> ELPNYLVTLPARLNFPSVQKVCLDLSPGYSDVKFTVTLETKDKTQKLLEYSGLKKRHLHCISFLVPPPAGGTEEVATIRVSGVGNNISFEEKKKVLIQRQGNGTFVQTDKPLYTPGQQVYFRIVTMDSNFVPVNDKYSMVELQDPNSNRIAQWLEVVPEQGIVDLSFQLAPEAMLGTYTVAVAEGKTFGTFSVEEYVLPKFKVEVVEPKELSTVQESFLVKICCRYTYGKPMLGAVQVSVCQKANTYWYREVEREQLPDKCRNLSGQTDKTGCFSAPVDMATFDLIGYAYSHQINIVATVVEEGTGVEANATQNIYISPQMGSMTFEDTSNFYHPNFPFSGKIRVRGHDDSFLKNHLVFLVIYGTNGTFNQTLVTDNNGLAPFTLETSGWNGTDVSLEGKFQMEDLVYNPEQVPRYYQNAYLHLRPFYSTTRSFLGIHRLNGPLKCGQPQEVLVDYYIDPADASPDQEISFSYYLIGKGSLVMEGQKHLNSKKKGLKASFSLSLTFTSRLAPDPSLVIYAIFPSGGVVADKIQFSVEMCFDNQVSLGFSPSQQLPGAEVELQLQAAPGSLCALRAVDESVLLLRPDRELSNRSVYGMFPFWYGHYPYQVAEYDQCPVSGPWDFPQPLIDPMPQGHSSQRSIIWRPSFSEGTDLFS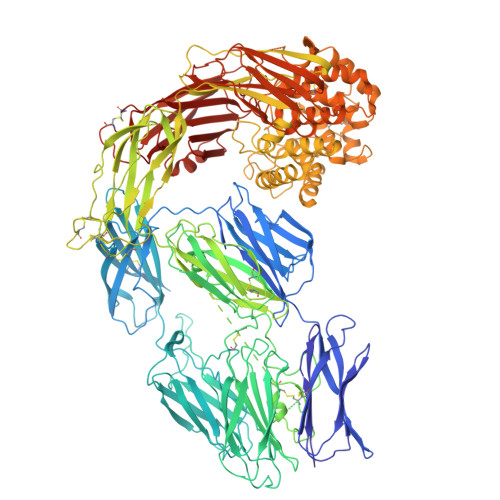FFRDVGLKILSNAKIKKPVDCSHRSPEYSTAMGAGGGHPEAFESSTPLHQAEDSQVRQYFPETWLWDLFPIGNSGKEAVHVTVPDAITEWKAMSFCTSQSRGFGLSPTVGLTAFKPFFVDLTLPYSVVRGESFRLTATIFNYLKDCIRVQTDLAKSHEYQLESWADSQTSSCLCADDAKTHHWNITAVKLGHINFTISTKILDSNEPCGGQKGFVPQKGRSDTLIKPVLVKPEGVLVEKTHSSLLCPKGKVASESVSLELPVDIVPDSTKAYVTVLGDIMGTALQNLDGLVQMPSGCGEQNMVLFAPIIYVLQYLEKAGLLTEEIRSRAVGFLEIGYQKELMYKHSNGSYSAFGERDGNGNTWLTAFVTKCFGQAQKFIFIDPKNIQDALKWMAGNQLPSGCYANVGNLLHTAMKGGVDDEVSLTAYVTAALLEMGKDVDDPMVSQGLRCLKNSATSTTNLYTQALLAYIFSLAGEMDIRNILLKQLDQQAIISGESIYWSQKPTPSSNASPWSEPAAVDVELTAYALLAQLTKPSLTQKEIAKATSIVAWLAKQHNAYGGFSSTQDTVVALQALAKYATTAYMPSEEINLVVKSTENFQRTFNIQSVNRLVFQQDTLPNVPGMYTLEASGQGCVYVQTVLRYNILPPTNMKTFSLSVEIGKARCEQPTSPRSLTLTIHTSYVGSRSSSNMAIVEVKMLSGFSPMEGTNQLLLQQPLVKKVEFGTDTLNIYLDELIKNTQTYTFTISQSVLVTNLKPATIKVYDYYLPDEQATIQYSDPCE> AEHCNAQMKTGPYKIKNLDITPPKETLQKDVEITIVETDYNENVIIGYKGYYQAYAYNGGSLDPNTRVEETMKTLNVGKEDLLMWSIRQQCEVGEELIDRWGSDSDDCFRDNEGRGQWVKGKELVKRQNNNHFAHHTCNKSWRCGISTSKMYSRLECQDDTDECQVYILDAEGNPINVTVDTVLHRDGVSMILKQKSTFTTRQIKAACLLIKDDKNNPESVTREHCLIDNDIYDLSKNTWNCKFNRCIKRKVEHRVKKRPPTWRHNVRAKYTEGDTATKGDLMHIQEELMYENDLLKMNIELMHAHINKLNNMLHDLIVSVAKVDERLIGNLMNNSVSSTFLSDDTFLLMPCTNPPAHTSNCYNNSIYK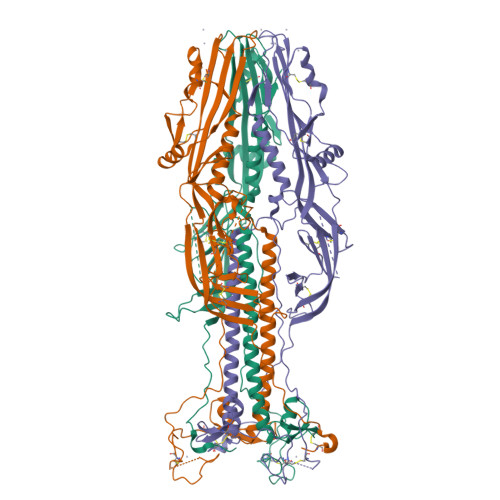EGRWVANTDSSQCIDFSNYKELAIDDDVEFWIPTIGNTTYHDSWKDASGWSFIAQQKSNLITTMENTKFGGVGTSLSDITSMAEGELAAKLTSFMFGHVVNFVIILIVILDYKDDDDK>[20x]TSVEFWQNIASGVGKWLRAIFAIAFWSSLILLTFYAIMTQVAPSKVFRLGALVDLIESVKTVLLGIFVFTASVTGIIAGVAAIANAFGASFAVSPIDVVNALIFQPIVDMVK

Here, we determine atomic structures by cryo-electron microscopy of three conjugative pili, two from hyperthermophilic archaea (Aeropyrum pernix and Pyrobaculum calidifontis) and one encoded by the Ti plasmid of the bacterium Agrobacterium tumefaciens, and show that the archaeal pili are homologous to bacterial mating pili. With structures for four bacterial conjugation pili (pED208, F, pKpQIL, and pTiC58 from A. tumefaciens) and two archaeal ones (A. pernix and P. calidifontis), it is clear that there is a common architecture for all and obvious homology, despite negligible sequence similarity. Each prokaryotic pilin subunit consists of two or three hydrophobic α-helices, with kinks appearing in some of the helices, such as in A. pernix and A. tumefaciens. Hence, pore diameters of all prokaryotic conjugative pili are sufficiently wide for the passage of ssDNA, but not dsDNA.

Cryo-EM analysis of the P. calidifontis filament preparation revealed pili, which following the reconstruction to 4.0 Å resolution, proved to be structurally similar to the CedA1 pili of A. pernix. While in the A. pernix filament the helical rise and twist per subunit were 3.6 Å and 76.5°, respectively, in the P. calidifontis filament these parameters were 5.0 Å and 74.2°. From the secondary structure and side-chain information present, we were able to determine the pilin identity directly from the cryo-EM map using DeepTracer-ID39 to be P. calidifontis protein Pcal_0765 (WP_011849449), which we name TedC (see below). Although TedC displays a similar fold to CedA1 from A. pernix, the two pilins are processed differently, with A. pernix pilin not being processed and the P. calidifontis pilin, similar to bacterial plasmid conjugative pilins, undergoing proteolytic cleavage. Notably, however, the mature P. calidifontis pilin contains an additional hydrophobic α-helix (α3) compared to pilins encoded by A. pernix and bacterial plasmids. In P. calidifontis the extended density could only be explained by a bipolar cyclic tetraether lipid. The cryo-EM map was good enough to identify the cyclic lipid as a glycerol dialkyl glycerol tetraether species (GDGT), a dominant membrane lipid in many hyperthermophilic archaea, including Pyrobaculum species, and we have modeled the simplest form, GDGT-0, into the cryo-EM density. Most of the pilin-lipid interaction network in the P. calidifontis pilus relies extensively on contacts with helix α1 in the asymmetric unit (ASU), but the lipid is sandwiched between α1 and α2 of a subunit in the neighboring ASU. Thus, the protein-lipid interaction stabilization relies heavily on hydrophobic interactions for P. calidifontis.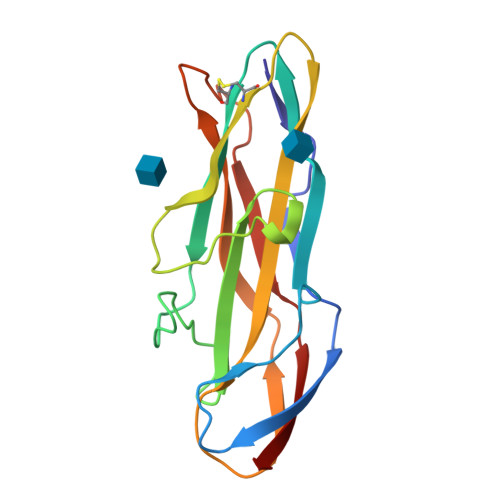>AVSFIGSTENDVGPSQGSYSSTHAMDNLPFVYNTGYNIGYQNANVWRISGGFCVGLDGKVDLPVVGSLDGQSIYGLTEEVGLLIWMGDTNYSRGTAMSGNSWENVFSGWCVGNYVSTQGLSVHVRPVILKRNSSAQYSVQKTSIGSIRMRPYNGSSAGSVQTTVNFSLNPFTLNDTVT[2x]>REQVKDSNGNPVKRGAKYFIQPAKSNGGGLVPAAINILPFCPLGITQTLLPYQPGLPVSFGYEPVIAGTDYIYTSTTINIEFRSEIWPVCNELSKLWAVDVSSSAAKEPAIIIGGERTAPNSLFKIEEATGAHTYKLTTSSGTVG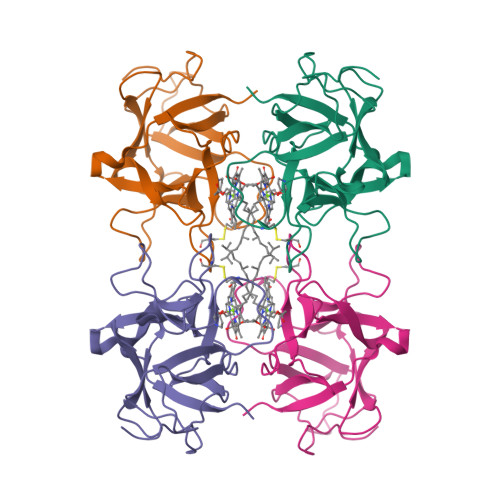TIPGPWLGAPQLIATNDDAKTLFVKFVKVDDDAT[2x]>LGSQYLDIVLLRGSSGLGFSIAGGTDNPHFDNDTSIYITKVIPGGAAEADG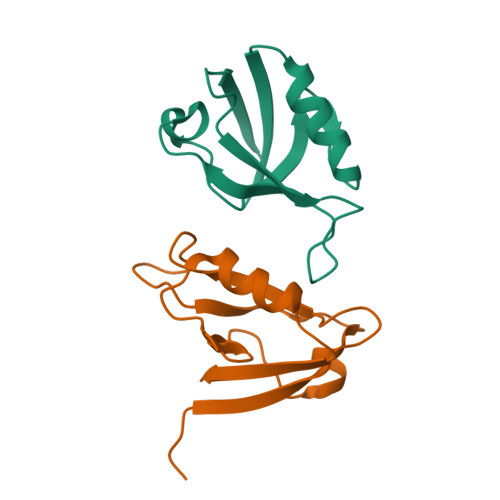RLKVYDTIVAVDDQLMEDVAHQVCVDALKSAGSEVKLRVKR[2x]2,6-dichloro-4-cyano-N-[2-({[(1R,2R)-2-fluorocyclopropyl]carbonyl}amino)pyridin-4-yl]benzamide | C17 H11 Cl2 F N4 O2 | 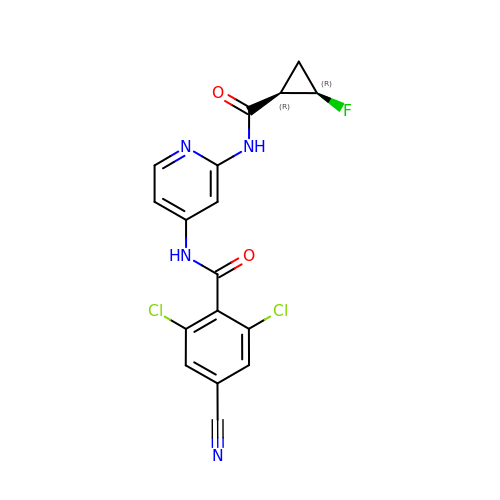TZBYGJGLZFYXII-GXFFZTMASA-N In this study, we identified and characterized a typhoid toxin-like A2B5 toxin, designated diarizonae toxin (DiaT), as a key virulence factor in Salmonella diarizonae. The DiaT genomic islet encodes two distinct B subunits, PltBd1 and PltBd2, which exhibit unique functional roles. Through genetic and functional analyses, we demonstrate that the heteropentameric assembly of PltBd1 and PltBd2 is essential for cytotoxicity, with our data suggesting PltBd1 facilitates toxin secretion and PltBd2 mediates host cell targeting. The holotoxin consists of a pentameric B subunit arrangement supporting a single PltA subunit, with the amphipathic C-terminal tail of PltA extending into the central pore formed by the B subunits.

To validate the structural insights from the cryo-EM map of the endogenously expressed DiaT holotoxin, we recombinantly expressed PltBd1 homopentameric holotoxin, PltBd2 homopentameric holotoxin, and PltBd1/PltBd2 heteropentameric holotoxin in E. coli. Cryo-EM analysis resolved these structures at resolutions of 3.05 Å, 2.61 Å, and 2.94 Å, respectively. Pore radius measurements confirmed that the PltBd1 homopentamer exhibits the smallest pore radius with significant distortion, while the PltBd2 homopentamer displays a larger and straighter pore. Further analysis of PltA’s interactions with distinct B subunits identified a critical hydrophobic interaction between Ile227 of PltA and Ile71 of PltBd2. Additionally, Tyr70 in PltBd1 forms stable polar interactions with Asn230 in PltA, contributing to the narrow, contracted pore structure, a feature absents in the PltBd2 homopentamer. All holotoxins demonstrated cytotoxic activity, but the PltBd2 homopentamer exhibited the highest potency, approximately threefold greater than the PltBd1/PltBd2 heteropentameric toxin (DiaT) and nearly 75-fold greater than the PltBd1 homopentamer. Despite its potent intoxication potential, the PltBd2 homopentameric holotoxin failed to restore cytotoxicity in the pltBd1 and pltBd2 double deletion strain complemented with pltBd2 alone. This suggests that PltBd2 homopentamers are likely unable to mediate extracellular secretion. The lower average dissociation constant exhibited by PltBd2 suggests a higher affinity for these glycans than PltBd1. Conversely, PltBd2 features a valine residue at the corresponding position (triangle, 6E and S12), limiting its binding capacity for Neu5Gc-terminated glycans, akin to PltB in typhoid toxin.

> MKKLILLTLIIASFDIYAIDFVYRVDPNPPDVIFRDGFSLLGYNRDLQQLISGRSCAGGSSDSRYIVTTSDINKTYAIARAYYSHSKFKGNLYRYKIRADNNFYSLTPSVNYLESQGGHFNAYEKSMIRLQSEYVSTLSILPENIQKAVALVYDSSTGQIKDGTSTINTDYVSISSVSNPGVIPFLPEPQANTQQRIDAFGSLISSCFSIYSVCQTHRGQKTEVYKMPFYDARPVIQFIISGN;>[5x]EWTGDSSINYYSDEVISDFHVGQFNRSAYFCIKTVKKSGEGTPIIACALSHDSKWIPSFNIMLEQARNFYITGHSIRVYVQPNVWSNKSFIEALSSNALVGLSSCSTSECFGPVKP> APVWGCASTRGRSAEMEDASAAVP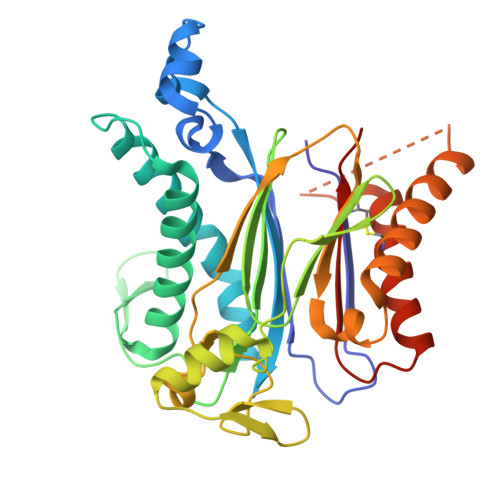RFADVPVRLLASRRDLDALGLDADALRLPAHLFGVFDGHGGAEVANYCRERIHVVLSAALARLGKNLGEMGEVDMKEHWDDVFTKCFQRVDDEVSGRVTRVVNGGGEVRSEPVTAENVGSTAVVALVCSSHVVVANCGDSRIVLCRGKEPVALSIDHKPDRKDERARIEAQGGKVIQWNGYRVSGLLAMSRSIGDRYLKPFVIPKPEVMVVPRAKDDDCLILASDGLWDVVSNEEACKVARRQILLWHKNNGAASPLSDEGEGSTDPAAQAAADYLMRLALKKGSEDNITVIVVDLKPRKKLKN> SMYAIRKIQFFYGPTDKKSYVGEEAGGRRELFKTRAEA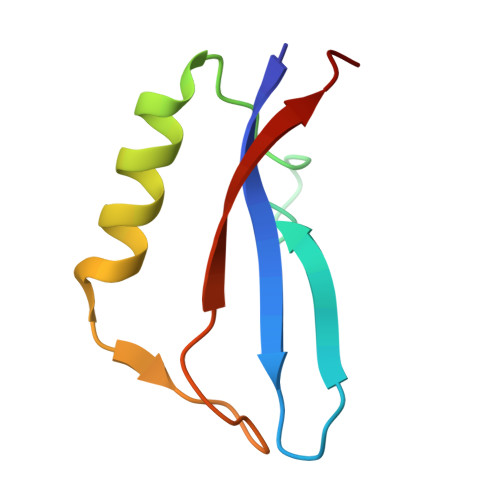QARIEDLEEGVYYLAHNESGRPDYKIVWVRGE>[6x]GSHMSQSLFSLAFGVGTQNRQEAWLEVFYALPLLKPSSEIVAAVAPILGYAAGNQALTFTSQQAYQLADALKGIDAAQSALLSRLAESQKPLVATLLAEDAAPSSTAEAYLKLHLLSHRLVKPHAVNLSGIFPLLPNVAWTNIGAVDLAELAELQLEARLKGKLLEVFSVDKFPKMTDYVVPAGVRIADTARVRLGAYIGEGTTVMHEGFVNFNAGTEGPGMIEGRVSAGVFVGKGSDLGGGCSTMGTLSGGGNIVISVGEGCLIGANAGIGIPLGDRNIVEAGLYITAGTKVALLDEQNALVKVVKARDLAGQPDLLFRRNSQNGAVECKTNKTAIELNEALHAHN

Pseudomonas aeruginosa is an opportunistic pathogen that causes persistent infections in humans. Randomized transposon mutagenesis screens had indicated several genes from the diaminopimelate (DAP) biosynthetic pathway to lysine in P. aeruginosa as essential, suggesting the corresponding gene products as potential targets for new antibacterial drugs. Dihydrodipicolinate synthase (DapA) catalyzes the first committed step of the DAP pathway, the condensation of L-aspartate-semialdehyde and pyruvate to 4-hydroxy-2,3,4,5-tetrahydro-L,L-dipicolinic acid, which is non-enzymatically dehydrated to yield L-2,3-diydrodipicolinate. Tetrahydrodipicolinate N-succinyltransferase (DapD) catalyses the transfer of the succinyl moiety of succinyl-CoA to the α-amino group of tetrahydrodipicolinate, the first committed step in the succinylase branch of the DAP biosynthesis pathway present in most Gram-negative bacteria and mycobacteria.

D-2-aminopimelic acid is not accepted as a substrate by PaDapD, but acts as a very weak inhibitor (IC50>20 mM). Eventually, these complexes could be prepared by soaking of monoclinic crystals of PaDapD in crystallisation liquor, where succinate had been replaced with either L- or D-2-aminopimelate. D-2-aminopimelate is bound to PaDapD in an extended conformation, well defined in the electron density maps. In five of the six active sites in the crystal asymmetric unit the interactions of this ligand are identical. The ε-carboxyl group of D-2-AP forms hydrogen bonds to the guanidinium groups of the two arginine residues Arg181 and Arg193, and the appropriate orientation of the side chains of these residues is ensured by a salt bridge to the side chain of Asp168. The head α-carboxyl group is anchored to the protein by hydrogen bonds to the main chain amino group of Ala226 and the side chain of Asn209. The α-amino group of the ligand is within hydrogen bonding distance to one of the carboxylate oxygen atoms of Glu221. In the active site located at the interface between subunits A and B, the binding mode of the ligand is different. While the tail carboxyl group and the carbon chain of D-2-AP interact in a similar manner with the enzyme as in the other subunits, the binding modes of the α-carboxyl- and α-amino groups are altered. We therefore suggest that binding of D-2-AP in a conformation incompatible with catalysis is the underlying basis for the discrimination of the enzyme against this stereoisomer of 2-aminopimelate.Enteroaggregative Escherichia coli is the primary cause of pediatric diarrhea in developing countries. They utilize aggregative adherence fimbriae (AAFs) to promote initial adherence to the host intestinal mucosa, promote the formation of biofilms, and mediate host invasion. Five AAFs have been identified to date and AAF/IV is amongst the most prevalent found in clinical isolates.

Here we present the X‐ray crystal structure of the AAF/IV tip protein HdaB at 2.0 Å resolution. It shares high structural homology with members of the Afa/Dr superfamily of fimbriae, which are involved in host invasion. We highlight surface exposed residues that share sequence homology and propose that these may function in invasion and also non‐conserved regions that could mediate HdaB specific adhesive functions.

>[2x]MGSHHHHHHGSADITLMNHKYMGNLLHDGVKLATGRIICQDTHSGFRVWINARQEGGGAGKYIVQSTEGPQHNLRIRIGGNGWSSFVEKGIQGVFNTIKEDASIFYIEVDGNQQVHPGKYLFSVSGECYIHMDNKQEFIPLCQAATITAQHTVEKLN> LRYDSTAER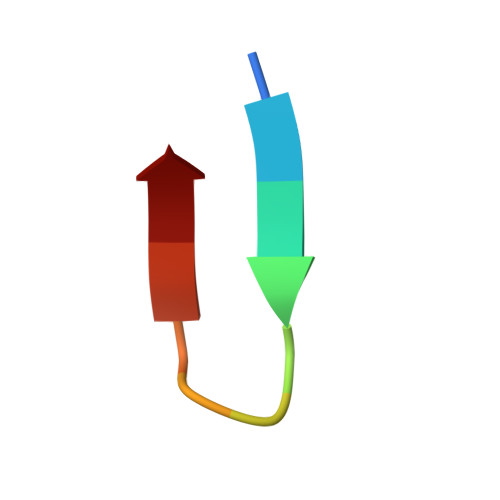LY4-(ACETYLAMINO)-3-AMINO 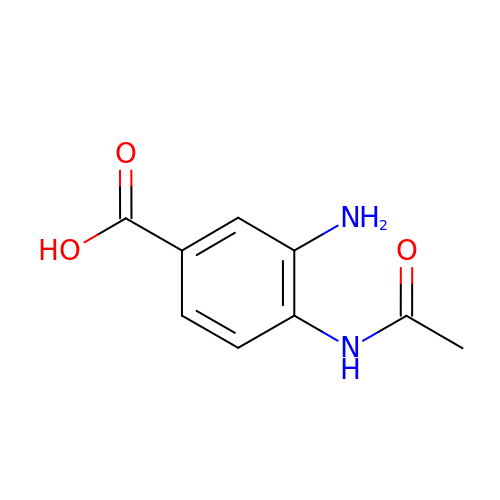BENZOIC ACID | C9 H10 N2 O3 | MJMLUICFHWSBQZ-UHFFFAOYSA-N In eukaryotes, the reverse transsulfuration pathway, which is composed of cystathionine β-synthase (CBS; EC 4.2.1.22) and cystathionine γ-lyase (CGL; EC 4.4.1.1), is involved in the biosynthesis of l-cysteine using l-serine and the sulfur atom in l-methionine. In the present study, we characterize the detailed enzymatic properties and determine the crystal structure of the putative CGL enzyme from L. plantarum SN35N to provide the structural basis for the reaction specificities. In summary, the L. plantarum CGL showed γ-lyase activity toward cystathionine and l-homocysteine to generate l-cysteine and H2S, respectively. In addition, it demonstrated β-lyase activity toward l-cystine, cystathionine, and l-cysteine to generate l-cysteine persulfide, l-homocysteine, and H2S, respectively.

Similarly, l-serine was also found as part of the external aldimine formed with PLP. In this case, a phosphate ion contained in the precipitant solution was found at the site for the binding to the distal carboxyl group of cystathionine. The α-carboxylate of the l-serine makes a strong interaction with the CGL enzyme, like that in cystathionine. In addition, the side-chain hydroxyl group may form a hydrogen bond with the side chain of Y97A (the distance is 3.1 ± 0.1 Å), although the electron density of the group is weak. In the crystal structure of the L. plantarum CGL complexed with l-serine as an analog of l-cysteine, the dihedral angle formed among carboxyl carbon, Cα, Cβ, and Oγ atoms in the PLP-bound l-serine is − 36° ± 17°, which seemed to be suitable for the β-lyase reaction. The conformation is likely caused by the hydrogen-bonding interaction between the Oγ atom and the hydroxyl group in the Y97A residue (3.1 ± 0.1 Å). The l-cysteine molecule is expected to be bound in a manner similar to l-serine, where the bound l-cysteine molecules undergo the β-lyase reaction to generate H2S. In addition, the side chain of the Glu320A residue is close to the Cγ and Sδ atoms of the bound cystathionine (4.2 ± 0.2 and 3.5 ± 0.3 Å, respectively) or the Oγ atom of the bound l-serine (4.1 ± 0.1 Å).

>MKFETQLIHGGISEDATTGATSVPIYMASTFRQTKIGQNQYEYSRTGNPTRAAVEALIATLEHGSAGFAFASGSAAINTVFSLFSAGDHIIVGNDVYGGTFRLIDAVLKHFGMTFTAVDTRDLAAVEAAITPTTKAIYLETPTNPLLHITDIAAIAKLAQAHDLLSIIDNTFASPYVQKPLDLGVDIVLHSASAYLGGHSDVIGGLVVTKTPALGEKIGYLQNAIGSILAPQESWLLQRGMKTLALRMQAHLNNAAKIFTYLKSHPAVTKIYYPGDPDNPDFSIAKQQMNGFGAMISFELQPGMNPQTFVEHLQVITLAESLGALESLIEIPALMTHGAIPRTIRLQNGIKDELIRLSVGVEASDDLLADLERGFASIQADLEHHHHHH[6x]N-[2-(4-{4-[2-amino-4-(difluoromethyl)pyrimidin-5-yl]-6-(morpholin-4-yl)-1,3,5-triazin-2-yl}piperazin-1-yl)-2-oxoethyl]-N-methyl-1-(prop-2-enoyl)piperidine-4-carboxamide | C28 H37 F2 N11 O4 | 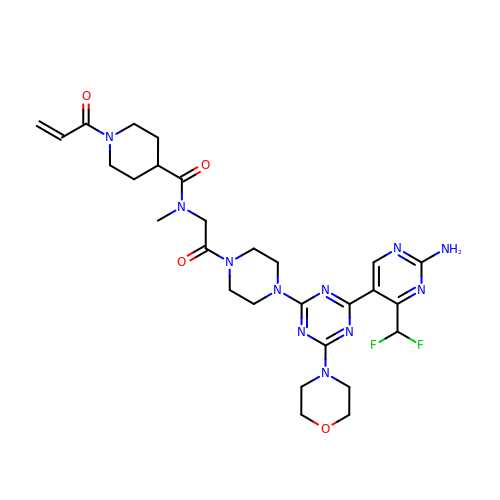DQXALALSPTWDRV-UHFFFAOYSA-N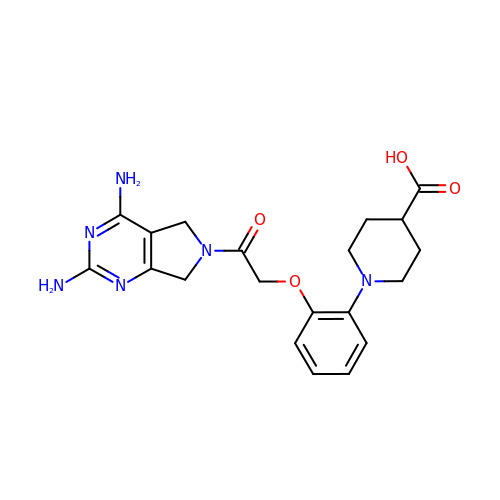1-{2-[2-(2,4-diamino-5,7-dihydro-6H-pyrrolo[3,4-d]pyrimidin-6-yl)-2-oxoethoxy]phenyl}piperidine-4-carboxylic acid | C20 H24 N6 O4 | GJSALIBRKRZNLE-UHFFFAOYSA-N>[4x]NLYFQGHMLEAAHLLEQMEYVFDEWIHLCNNPHATERAAMIFVHQLHSVQLVTNRDEFLLFLRHALDKSVERFEQGIHSGASIAESFQAVEALVKLIIIFVKSHQDSEDKDPSAAVAFMDSILALGVLVANSHHVKRGENFNQRVFYRFFALLLHEVGLLAGHFSKSHYEQIILNFAARLFDMRPNLLPGFACAWAGLVSHRAFLPVILGLPDEKGWAPFTKLLEQFLGCVGEL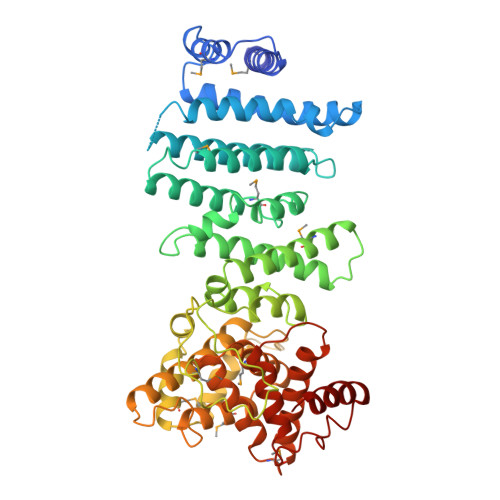VKTFTVSSLGKEMYHAALKILIVLQHDFPIYLDKFRVQLCQSLPLHATQLVNLILAAIPPNCNSLADPFQAGLKVDKIPDMKERPPTAFDSAGLLREAGLLDILERMLQNGPSEDGVAQINHAINKSDGESTSFGYVPLGVNRRLIDAVVARFAEFAINRASSRSDSAIFVAGANDIKTLQMLVTEVSPEARYYLVSSMVNELRYPNAYTNYFSQALLDIFGHDMSDPEENLVREQIVRVLLERVLGYWPQPWGLIITILELLKNDKYLFFELPFIKATPEVAERFTALARSAA>[2x]MAMDVTRSQA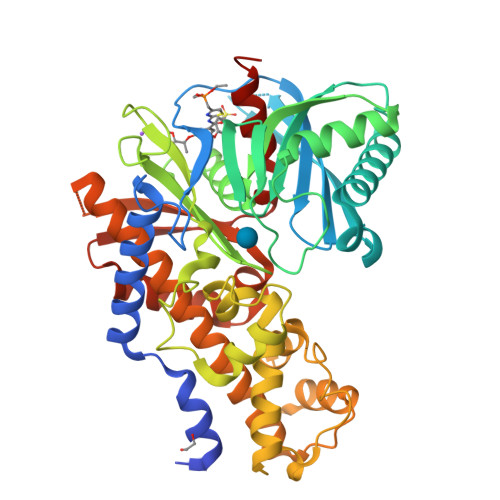QTALTLVEQILAEFQLQEEDLKKVMRRMQKEMDRGLRLETHEEASVKMLPTYVRSTPEGSEVGDFLSLDLGGTNFRVMLVKVGEGEEGQWSVKTKHQMYSIPEDAMTGTAEMLFDYISECISDFLDKHQMKHKKLPLGFTFSFPVRHEDIDKGILLNWTKGFKASGAEGNNVVGLLRDAIKRRGDFEMDVVAMVNDTVATMISCYYEDHQCEVGMIVGTGCNACYMEEMQNVELVEGDEGRMCVNTEWGAFGDSGELDEFLLEYDRLVDESSANPGQQLYEKLIGGKYMGELVRLVLLRLVDENLLFHGEASEQLRTRGAFETRFVSQVESDTGDRKQIYNILSTLGLRPSTTDCDIVRRACESVSTRAAHMCSAGLAGVINRMRESRSEDVMRITVGVDGSVYKLHPSFKERFHASVRRLTPSCEITFIESEEGSGRGAALVSAVACKKACMLGQ> MESKGASSCRLLFCLLISATVFRPGLGWYTVNSAYGDTIIIPCRLDVPQNLMFGKWKYEKPDGSPVFIAFRSSTKKSVQYDDVPEYKDRLNLSENYTLSISNARISDEKRFVCMLV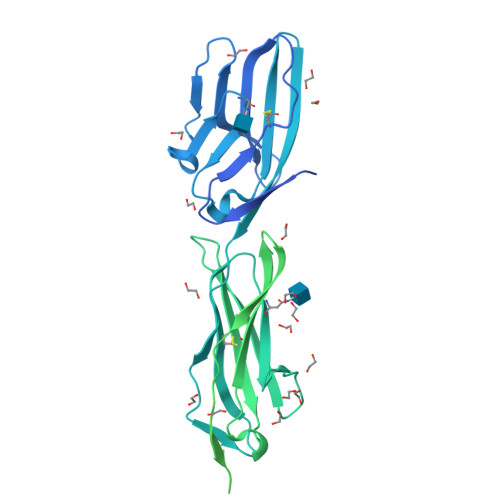TEDNVFEAPTIVKVFKQPSKPEIVSKALFLETEQLKKLGDCISEDSYPDGNITWYRNGKVLHPLEGAVVIIFKKEMDPVTQLYTMTSTLEYKTTKADIQMPFTCSVTYYGPSGQKTIHSEQAVFDIYYPTEQVTIQVLPPKNAIKEGDNITLKCLGNGNPPPEEFLFYLPGQPEGIRSSNTYTLTDVRRNATGDYKCSLIDKKSMIASTAITVHYLDLSLNPSGEVTRQIGDALPVSCTISASRNATVVWMKDNIRLRSSPSFSSLHYQDAGNYVCETALQEVEGLKKRESLTLIVEGKPQIKMTKKTDPSGLSKTIICHVEGFPKPAIQWTITGSGSVINQTEESPYINGRYYSKIIISPEENVTLTCTAENQLERTVNSLNVSAISIPEHDEADEISDENREKVNDQAKLIVGIVVGLLLAALVAGVVYWLYMKKSKTASKHVNKDLGNMEENKKLEENNHKTEA CG30463 is predicted to encode a ppGalNAcT/PGANT, which is an O-glycosyltransferase responsible for the post-translational addition of the sugar N-acetylgalactosamine (GalNAc) to proteins, a modification typically found on mucins and other secreted and membrane-bound proteins. ppGalNAcTs are type II membrane proteins that belong to the CAZy family GT2731. Interestingly, we found two distinct Drosophila cDNA clones emanating from the CG30463 gene, differing only in a ~30 amino acid region (the α subunit) of the lectin domain. Comparison of these clones to genomic sequence data revealed that they represent splice variants of exon 8. This splicing event generates an α subunit with a net positive charge (isoform A, containing exon 8A) or a net negative charge (isoform B, containing exon 8B). PGANT9A and PGANT9B adopt the canonical ppGalNAcT tertiary structure where a ~10 amino acid flexible linker connects the N-terminal catalytic domain to the C-terminal lectin domain.

PGANT9B crystallizes with 2 molecules per asymmetric unit, but density for UDP, Mn2+, or a peptide is not present in the active site under these crystallization conditions. The active site residue Asp 301 is misaligned, and the active site loop is disordered. The variable loop in PGANT9B adopts a similar conformation as the loop in PGANT9A, except that negatively charged residues Glu 538, Glu 541, Glu 542, and Glu 543 are clustered at the region of the loop near the active site to form a negatively charged patch. Another charged region is evident in the electrostatic potential map, where residues including Asp 535 and Glu 550 form a distinct negatively charged patch on the surface of the lectin domain. Thus, both enzymes have two distinct charged patches in their lectin domain formed by the α-subunit that results in preferences to recruit either negatively (PGANT9A) or positively (PGANT9B) charged substrates to the active site for catalysis. In PGANT9A and PGANT9B, the loop is closer to the active site than in the other ppGalNAcTs. In agreement with what was seen in cell culture, in vitro enzyme assays revealed that both PGANT9A and PGANT9B are capable of glycosylating the neutral T-rich peptide derived from the T-rich region (PPTQQSTTQPPCTTS), but only PGANT9B was able to efficiently glycosylate the positively charged PTTTK peptide derived from the PTTTK repetitive region (PTTTKPTTTKPTTTK).

>GGGGGPGELGKPVRLPKEMSDEMKKAVDDGWTKNAFNQYVSDLISVHRTLPDPRDAWCKDEARYLTNLPKTDVIICFHNEAWTVLLRTVHSVLDRSPEHLIGKIILVDDYSDMPHLKRQLEDYFAAYPKVQIIRGQKREGLIRARILGANHAKSPVLTYLDSHCECTEGWLEPLLDRIARNSTTVVCPVIDVISDETLEYHYRDSGGVNVGGFDWNLQFSWHPVPERERKRHNSTAEPVYSPTMAGGLFSIDREFFDRLGTYDSGFDIWGGENLELSFKTWMCGGTLEIVPCSHVGHIFRKRSPYKWRSGVNVLKKNSVRLAEVWMDEYSQYYYHRIGNDKGDWGDVSDRRKLRNDLKCKSFKWYLDNIYPELFIPGDSVAHGEIANVPNGMCLDAKEKSEEETPVSIYECHGQGGNQYWMLSKAGEIRRDDSCLDYAGKDVTLFGCHGGKGNQFWTYRENTKQLHHGTSGKCLAISESKDKLLMEECSASLSRQQWTLENYDSSKL[2x]> MAVLKIISWNVNGLRA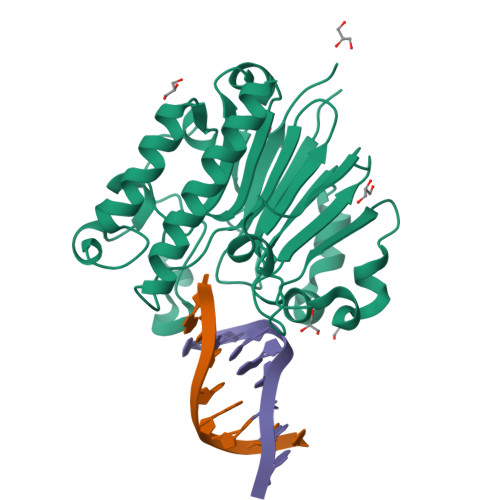VHRKGFLKWFMEEKPDILCLQEIKAAPEQLPRKLRHVEGYRSFFTPAERKGYSGVAMYTKVPPSSLREGFGVERFDTEGRIQIADFDDFLLYNIYFPNGKMSEERLKYKLEFYDAFLEDVNRERDSGRNVIICGNFNTAHREIDLARPKENSNVSGFLPVERAWIDKFIENGYVDTFRMFNSDPGQYTWWSYRTRARERNVGWRLDYFFVNEEFKGKVKRSWILSDVMGSDHCPIGLEIELLEHHHHHH>[2x]METRPLVIIGAGPAGLSAAVYTARAGIPTLVFGSAPKVAGDYDIDNYFGF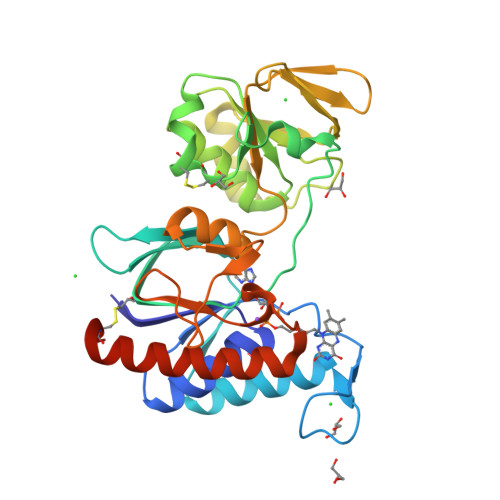DETITGRELIERGRRQAERFGAVLRDDRILGLHHGDDGGFRITTEAGETAACAIILATGVSRVRPGISNIADYEGKGVSYCVSCDGFFYRGLRVKVLGEGVFAANQALELLHYTPHVSICTQGKAASITPEFMTRLDEAGIAVDDRKIASLEGTPALSVLRYEDGSTEEAQGLFIAMGEASSLDFAYTLGVERNGVFLGADSDQRTNIPGVFAAGDCTGGFLQIAVAVGEGAKAARAAISYIKEECPFATSRRNTTTES Riboswitches are cis-acting gene regulatory elements that are mostly found in bacteria (Lee et al., 2009). They are located in the 5′ untranslated region (UTR) of mRNAs and consist of an aptamer domain that binds the ligand, and an expression platform that controls the expression of the downstream gene. The GRA was derived by a point mutation from the guanine riboswitch (C74U) (Gilbert et al., 2006b). As a result, the specificity of the guanine riboswitch was altered to be adenine responsive, thus generating a new adenine riboswitch (GRA).

Compounds 24 and 28 are both based upon scaffolds that were not previously observed to bind to adenine-sensing riboswitches. With binding affinities of 370 and 650 μM, they are rather weak ligands. Compound 24 hydrogen bonds with the bases of U51 and U74, the ribose of U22 and water molecule W2329 which is located in an equivalent position to W364 in the docking calculations. The observed and the predicted binding mode agreed within experimentally error (rmsd = 0.21 Å). Superimposing the binding modes of the ligands 2 and 24 reveals that both compounds have a similar arrangement of hydrogen-bond donor and acceptor groups with respect to U51 and U47. However, 24 forms an additional hydrogen bond to the ribose of U47 but is in turn lacking a hydrogen-bond donor group to interact with the 4-oxo group of the base of U74. The difference in the binding affinities of 2,6-diaminopurine (1) and 2-aminopurine (3) suggests that the formation of the hydrogen bond to U74 can lead to a 30-fold improvement in binding affinity (Gilbert et al., 2006b). Apparently, the additional hydrogen bond formed by 24 with the ribose can not compensate for the loss of this important hydrogen bond. Nevertheless, retrieving the ligands 24 and 28 underlines the power of molecular docking to discover hits that are structurally unrelated to known ligands.

> GGACAUAUAAUCGCGUGGAUAUGGCACGCAAGUUUCUACCGGGCACCGUAAAUGUCCGAUUAUGUCC>[4x]AAVTQSPRNKVAVTGEKVTLSCQQTNNHNNMYWYRQDTGHGLRLI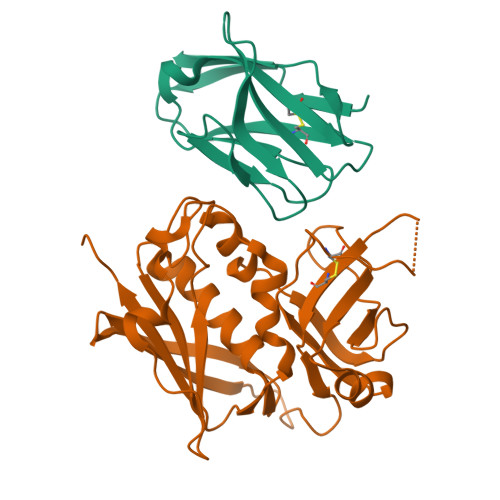HYSYGAGSTEKGDIPDGYKASRPSQEQFSLILESATPSQTSVYFCASGGGGTLYFGAGTRLSVL;>[4x]ESQPDPMPDDLHKSSEFTGTMGNMKYLYDDHYVSATKVKSVDKFLAHDLIYNISDKKLKNYDKVKTELLNEDLAKKYKDEVVDVYGSNYYVNCYFSSKDNKASTWHGKTCMYGGITKHEGNHFDNGNLQNVLVRVYENKRNTISFEVQTDKKSVTAQELDIKARNFLINKKNLYEFNSSPYETGYIKFIENNGNTFWYDMMPAPGDKFDQSKYLMMYNDNKTVDSKSVKIEVHLTTKNG>SRAPAPATPHAPDHSPAPNSPTLTRPPEGPKFPRVKNWELGSITYDTLCAQSQQDGPCTPRRCLGSLVLPRKLQTRPSPGPPPAEQLLSQARDFINQYYSSIKRSGSQAHEERLQEVEAEVASTGTYHLRESELVFGAKQAWRNAPRCVGRIQWGKLQVFDARDCSSAQEMFTYICNHIKYATNRGNLRSAITVFPQRAPGRGDFRIWNSQLVRYAGYRQQDGSVRGDPANVEITELCIQHGWTPGNGRFDVLPLLLQAPDEAPELFVLPPELVLEVPLEHPTLEWFA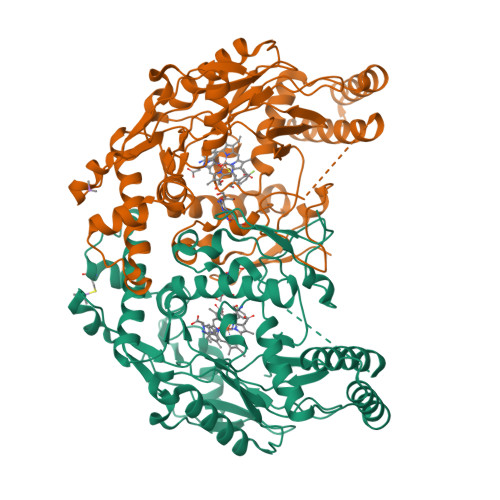ALGLRWYALPAVSNMLLEIGGLEFSAAPFSGWYMSTEIGTRDLCDPHRYNILEDVAVCMDLDTRTTSSLWKDKAAVEINLAVLHSFQLAKVTIVDHHAATVSFMKHLDNEQKARGGCPADWAWIVPPISGSLTPVFHQEMVNYILSPAFRYQPDPW[2x]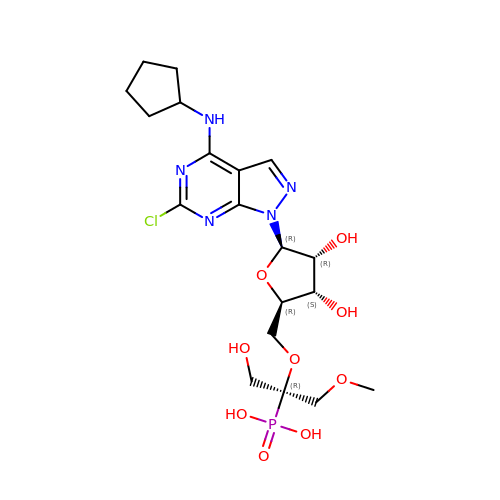6-chloro-N-cyclopentyl-1-{5-O-[(2R)-1-hydroxy-3-methoxy-2-phosphonopropan-2-yl]-beta-D-ribofuranosyl}-1H-pyrazolo[3,4-d]pyrimidin-4-amine | C19 H29 Cl N5 O9 P | BQCRMLSBGAKPFW-RTPDKIPNSA-N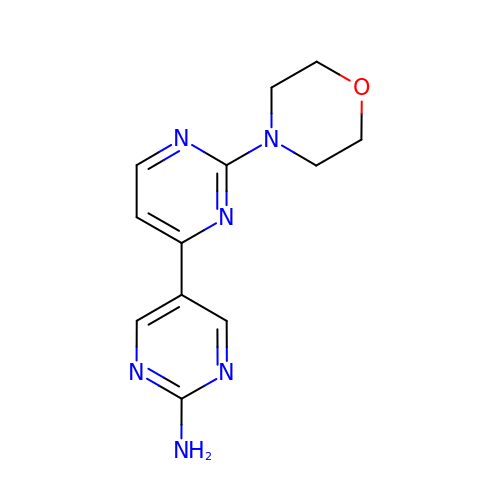2-(morpholin-4-yl)[4,5'-bipyrimidin]-2'-amine | C12 H14 N6 O | WCSNDONKXWSCEI-UHFFFAOYSA-N> SVDDEPIRLPNPMIGFGVPNEPGLITHRSLPELARGPPFFYYENVALTPKGVWETISRHLFEIPPEFVDSKYFCVAARKRGYIHNLPINNRFQIQPPPKYTIHDAFPLSKRWWPEWDKRTKLNCILTRTGSAQLTNRIRVALEPYNEEPEPPKHVQRYVIDQCKKWNLVWVGKNKAAPLEPDEMESILGFPKNHTRGGGMSRTERFKSLGNSFQVDTVAYHLSVLKPIFPHGINVLSLFTGIGGGEVALHRLQIKMKLVVSVEISKVNRNI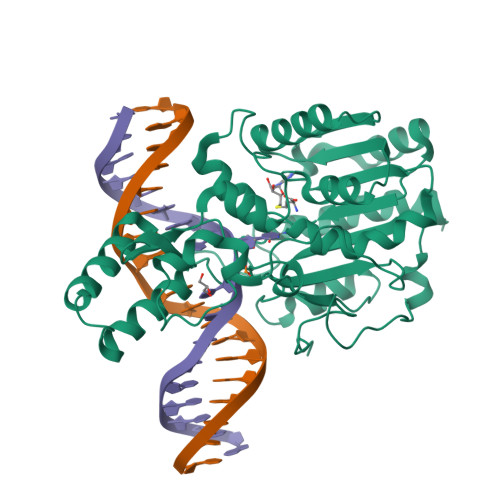LKDFWEQTNQTGELIEFSDIQHLTNDTIEGLMEKYGGFDLVIGGSPCNNLAGGNRVSRVGLEGDQSSLFFEYCRILEVVRARMRGS>[4x]MLHQLTLAEIARALADKQFSAEELTRTLLGRIRQLDPQLNSFISITDDLAIAQAKAADERRANGENGALLGAPIAHKDLFCTQGVRTSCGSKMLDNFVSPYDATVVEKLTAAGAVTLGKLNMDEFAMGSSNQSSHYGAVKNPWSLDRVPGGSSGGSAAAVAARLLPAATGTDTGGSIRQPAALTNLTGIKPTYGRVSRWGMIAYASSLDQGGPLARTAEDCALMLGVMAGFDPKDSTSVEQPVDDYLAALQKPLSGLRIGLPREYFGAGLDSRIADAVLAVVEELKTLGATVKDISLPNMQHAIPAYYVIAPAEASSNLSRFDGVRYGYRCDAPQNLEDLYKRSRAEGFGSEVKNRIMVGTYALSAGYYDAYYLQAQKIRRLIKNDFVSAFAEVDVILGPTTPNPAWKIGEKNDDPVSQ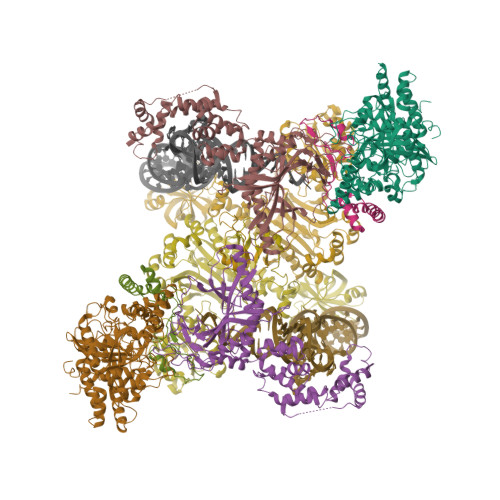YLEDIYTITANLAGLPGLSMPAGFVDGLPVGVQLLAPYFQEGRLLNVAHQYQQVSDWHTRTPAGF;>MQWETVIGLEIHAQLATQSKIFSGSSTAFGAAPNTQASLVDLAMPGTLPVLNEEAVRMACLFGLAIDARIDRQNVFARKNYFYPDLPKGYQTSQMDHPIVGKGHLDITLEDGTTKRIGITRAHLEEDAGKSLHEDFQGMSGIDLNRAGTPLLEIVSEPDIRSAKEAVAYVKAIHALVRYLGICDGNMAEGSLRCDCNVSVRPKGQAEFGTRAEIKNVNSFRFIEKAINHEIQRQIELIEDGGKVVQETRLYDPNKDETRSMRGKEEANDYRYFPCPDLLPVVIEPEYLAKLREQLPELPVQKRERFESQYGLSAYDASVLSASREMADYFEKVQGICGDAKLAANWVMVELGSLLNKDGLEIEQSPVSAEQLGGMILRIKDNTISGKLAKMVFEAMANGEGSAXXXXXXXXXXXXXXXXXXXXXXXXXXXXXXXXXXXXXXXXXXXXXXXXXXXXXXXXXXXXXXXXXXXXXXXXXXXXXX[4x];>MGHHHHHHMALERSDVEKIAHLARLGLSEADLPRTTETLNNILGLIDQMQAVDTSGVEPLAHPLEATQRLRPDAVTETDHRDAYQTIAPAVEEGLYLVPKVIES[4x];>[4x]MGHHHHHHMMRSHYCGQLNESLDGQEVTLCGWVHRRRDHGGVIFLDVRDREGLAQVVFDPDRAETFAKADRVRSEFVVKITGKVRLRPEGARNPNMASGSIEVLGYELEVLNQAETPPFPLDEYSDVGEETRLRYRFIDLRRPEMAAKLKLRARITSSIRRYLDDNGFLDVETPILGRPTPEGARDYLVPSRTYPGHFFALPQSPQLFKQLLMVAGFDRYYQIAKCFRDEDLRADRQPEFTQIDIETSFLDESDIIGITEKMVRQLFKEVLDVEFDEFPHMPFEEAMRRYGSDKPDLRIPLELVDVADQLKEVEFKVFSGPANDPKGRVAALRVPGAASMPRSQIDDYTKFVGIYGAKGLAYIKVNERAKGVEGLQSPIVKFIPEANLNVILDRVGAVDGDIVFFGADKAKIVCDALGALRIKVGHDLKLLTREWAPMWVVDFPMFEENDDGSLSALHHPFTSPKCTPAELEANPGAALSRAYDMVLNGTELGGGSIRIHDKSMQQAVFRVLGIDEAEQEEKFGFLLDALKYGAPPHGGLAFGLDRLVMLMTGASSIREVIAFPKTQSAGDVMTQAPGSVDGKALRELHIRLREQPKAE> TEIEHLVQSVCKSYRETCQLRLEDLLRQRSNIFSREEVTGYQRKSMWEMWERCAHHLTEAIQYVVEFAKRLSGFMELCQNDQIVLLKAGAMEVVLVRMCRAYNADNRTVFF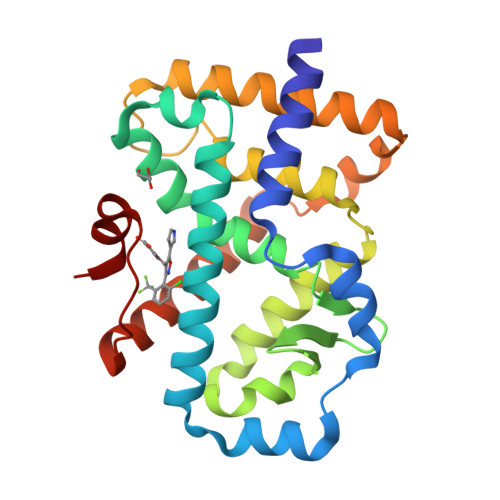EGKYGGMELFRALGCSELISSIFDFSHSLSALHFSEDEIALYTALVLINAHRPGLQEKRKVEQLQYNLELAFHHHLHKTHRQSILAKLPPKGKLRSLCSQHVERLQIFQHLHPIVVQAAFPPLYKELFS>[6x]GSMTTVMNDKHPTPDPAEDNAFFPSAYSLSQFTA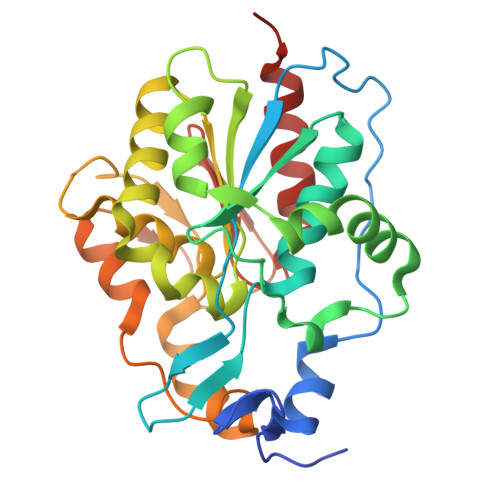SKSDLSGAHYPTPYQGGRWKILVVGADERYLMMDNGTFFSTGNHPVETLLPMYHLDKAGFSFDIATLSGNPVKFEWWAMPREDQEVNGLYSKYQSSFRQPLKLSDVIETALGEDSDYIGVFIPGGHGALMGLPDSQEVKAVLQWAMKQNKFIISLCHGPAAFLAVGDDPLFAGYKIVAFPDEMDAQTPSIGYMPGHLTWKFGEQLQAIGFELLNTGISGQVFQDRKMLTGDSPLAGNALGQLAAKALLAEVEQK> GAMGSMGTRDDEYDYLFKVVLIGDSGVGKSNLLSRFTRNEFNLESKSTIGVEFATRSIQVDGKTIKAQIWDTAGLERYRAITSAYYRGAVGALLVYDIAKHLTYENVERWLKELRDHADSNIVIMLVGNKSDLRHLRAVPTDEARAFAEKNGLSFIET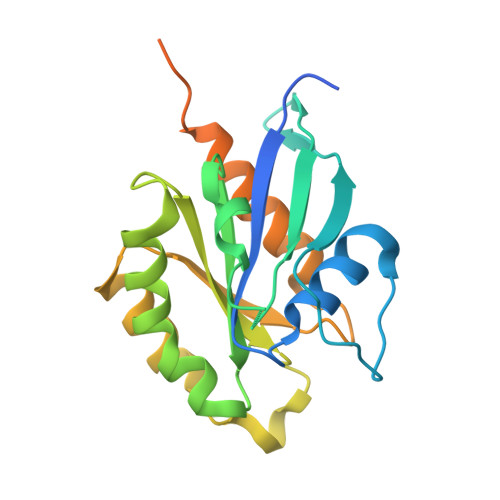SALDSTNVEAAFQTILTEIYRIVSQKQMSDRRENDMSPSNNVVPIHVPPTTENKPKVQCCQNI> MGYNKSLRYSRHDGTSCVIDNHHLKSLGAVLNDVRRKKDRIREAEYEPIIDIADQYMVTEDPFRGPGKNVRITLFKEIRRVHPDTMKLVCNWSGKEFLRETWTRFISEEFPITTDQEIMDLWFELQLRPMHPNRCYKFTMQYALG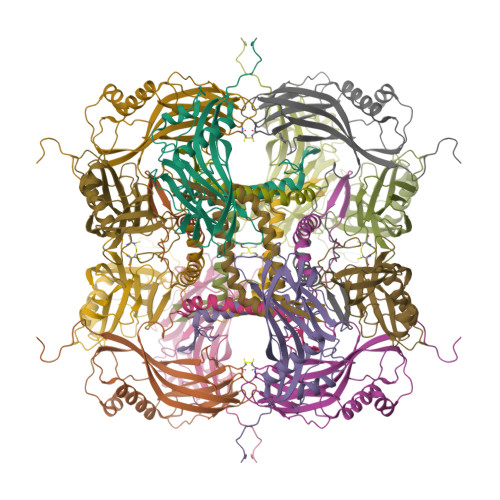AHPDYVAHDVIRQQDPYYVGPNNIERINLSKKGFAFPLTCLQSVYNDNFERFFDDVLWPYFYRPLVYVGTTSAEIEEIMIEVSLLFKIKEFAPDVPLFTGPAY>MGLSTATKRLGHLLPQSSILFVCDVQEVFRGLTFQLPTVIHSTNTMVSAAKLLNLPVVVTTQYGSRLGSTVSEISKNLENVNDVKIFDKMKFSMLVPEVEHHLTSNMPQRKSVLLCGIETHVCVLQTCLDLLDKGYDVHVVSDAVSSSTSYNRSMALERMRQSGAYITSVESAIFQLANDASNPEFKIISKLIK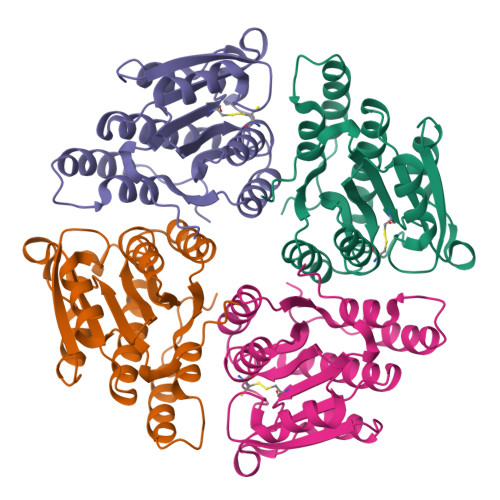EHLKVGNGFDTGALI[16x]2-[(methylsulfonyl)methyl]-1H-benzimidazole | C9 H10 N2 O2 S | 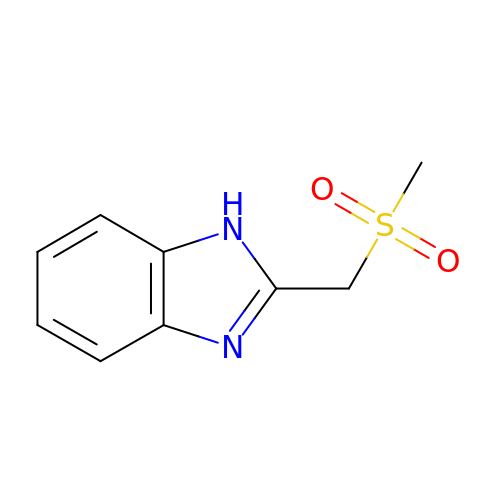WCWTYTQSZZWNEW-UHFFFAOYSA-N> MIDGAEVSVSRGKNNPF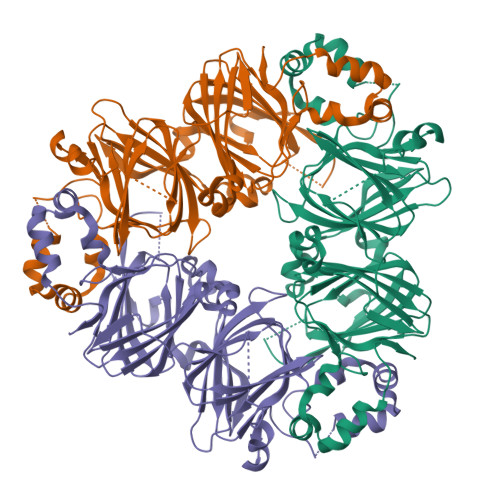YFNSDRWFHTLFRNQFGHLRVLQRFDQRSKQMQNLENYRVVEFNSKPNTLLLPHHADADFLLVVLNGRAVLTLVNPDGRDSNILEQGHAQKIPAGTTFFLVNPDDEENLRIIKLAVPVNNPHRFQDFFLSSTEAQQSYLQGFSKNILEASFDSDIKEISRVLFGEEGQQQQQGQESQQEGVIVELKREQIRELTKHAKSSSKKSLSSEDQPFNLRNQKPIYSNKLGRWFEITPEKNPQLRDLDMFIRSVDMKEGSLLLPHYNSKAIVILVINEGKANIELVGQREQQKQQEEQEESWEVQRYRAELSEDDVFIIPATYPVAINATSNLNFFAFGINAENNQRNFLAGEKDNVISEIPTEVLDVTFPASGEKVQKLIKKQSESQFVDAQPEQQEREEARKGGKGPFVY>[3x]GAMDQRMYSRRSLYHTRTKDLKDFIRVHRLPKALAQRMLECFQTTWSVNNGIDVSELLKDFPDELRADIAMHLNKE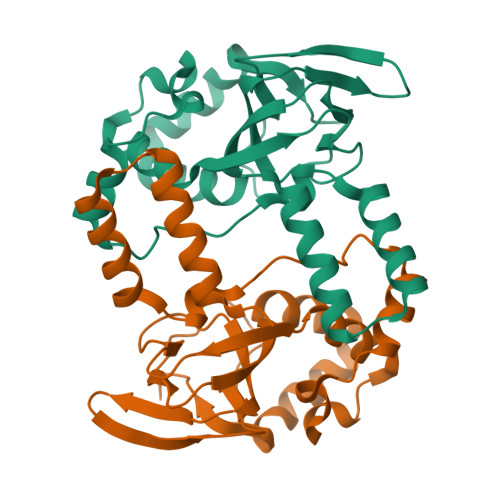LLQLPLFESASRGCLRSLSLIIKTSFCAPGEFLIRQGDALQAIYFVCSGSMEVLKDNTVLAILGKGDLIGSDSLTKEQVIKTNANVKALTYCDLQYISLKGLREVLRLYPEYAQKFVSEIQHDLTYNLREGSGADL>HHHHHHHHAPLLLYANRRDLRLVDATNGKENATIVVGGLEDAAAVDFVFSHGLIYWSDVSEEAIKRTEFNKTESVQNVVVSGLLSPDGLACDWLGEKLYWTDSETNRIEVSNLDGSLRKVLFWQELDQPRAIALDPSSGFMYWTDWGEVPKIERAGMDGSSRFIIINSEIYWPNGLTLDYEEQKLYWADAKLNFIHKSNLDGTNRQAVVKGSLPHPFALTLFEDILYWTDWSTHSILACNKYTGEGLREIHSDIFSPMDIHAFSQQRQPNATNPCGIDNGGCSHLCLMSPVKPFYQCACPTGVKLLENGKTCKDGATELLLLARRTDLRRISLDTPDFTDIVLQLEDIRHAIAIDYDPVEGYIYWTDDEVRAIRRSFIDGSGSQFVVTAQIAHPDGIAVDWVARNLYWTDTGTDRIEVTRLNGTMRKILISEDLEEPRAIVLDPMVGYMYWTDWGEIPKIERAALDGSDRVVLVNTSLGWPNGLALDYDEGKIYWGDAKTDKIEVMNTDGTGRRVLVEDKIPHIFGFTLLGDYVYWTDWQRRSIERVHKRSAEREVIIDQLPDLMGLKATNVHRVIGSNPCAEENGGCSHLCLYRPQG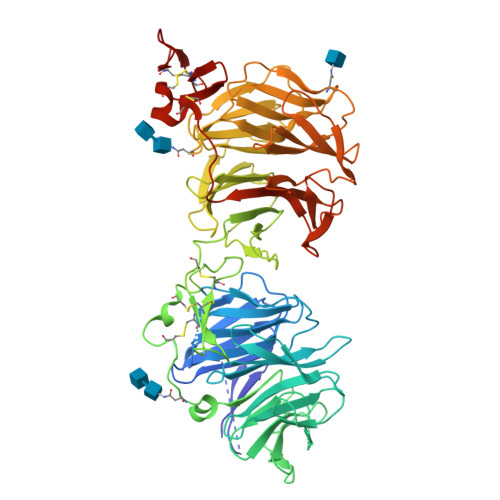LRCACPIGFELISDMKTCIVP[2x]(2~{S})-2-[[(2~{S})-6-[(4-fluorophenyl)amino]-1-oxidanyl-1,6-bis(oxidanylidene)hexan-2-yl]carbamoylamino]pentanedioic acid | C18 H22 F N3 O8 | 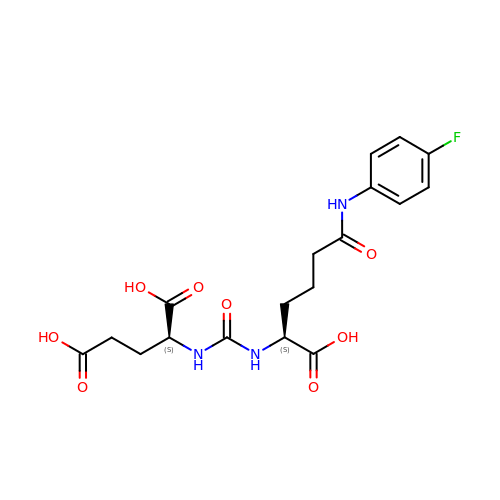CKNIHKIYCHYOOG-STQMWFEESA-N> MIQGVIQKIAGPAVIAKGMLGARMYDICKVGEEGLVGEIIRLDGDTAFVQVYEDTSGLKVGEPVVSTGLPLAVELGPGMLNGIYDGIQRPLERIREKTGIYITRGVVVHALDREKKWAWTPMVKPGDEVRGGMVLGTVPEFGFTHKILVPPDVRGRVKEVKPAGEYTVEEPVVVLEDGTELKMYHTWPVRRARPVQRKLDPNTPFLTGMRILDVLFPVAMGGTAAIPGPFGSGKTVTQQSL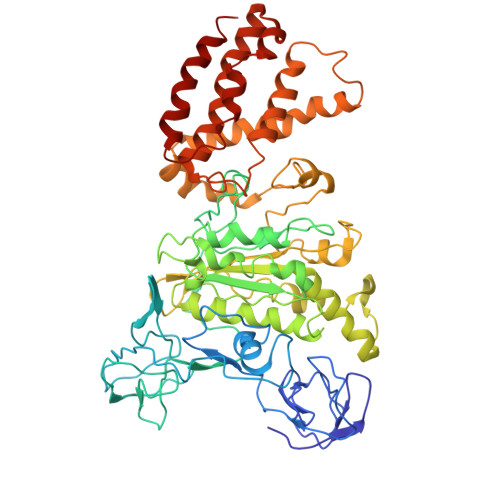AKWSNADVVVYVGCGERGNEMTDVLVEFPELTDPKTGGPLMHRTVLIANTSNMPVAAREASIYVGVTIAEYFRDQGFSVALMADSTSRWAEALREISSRLEEMPAEEGYPPYLAARLAAFYERAGKVITLGGEEGAVTIVGAVSPPGGDMSEPVTQSTLRIVGAFWRLDASLAFRRHFPAINWNGSYSLFTSALDPWYRENVAEDYPELRDAISELLQREAGLQEIVQLVGPDALQDAERLVIEVGRIIREDFLQQNAYHEVDAYCSMKKAYGIMKMILAFYKEAEAAIKRGVSIDEILQLPVLERIGRARYVSEEEFPAYFEEAMKEIQGAFKAL>GSHMSNTQTVLPFTGLNTPSGVAVDSAGTVYVTDHGNNRVVKLAAGSNTQTVLPFTGLNTPH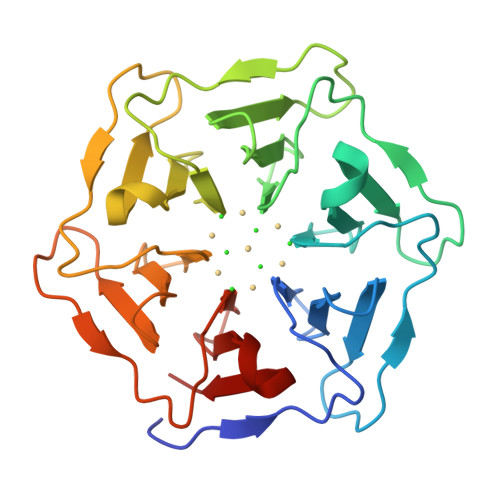GVAVDSAGTVYVTDHGNNRVVKLAAGSNTQTVLPFTGLNTPSGVAVDSAGTVYVTDHGNNRVVKLAAGSNTQTVLPFTGLNTPHGVAVDSAGTVYVTDHGNNRVVKLAAGSNTQTVLPFTGLNTPSGVAVDSAGTVYVTDHGNNRVVKLAAGSNTQTVLPFTGLNTPHGVAVDSAGTVYVTDHGNNRVVKLAAG[2x]>[3x]MNVASRVVVNADRVKGTINRNIYGHFSEHLGRCIYEGLWVGEDSPIPNTNGIRNDVLEALKQMKIPVLHWPGGCFADEYHWKDGVGPREKRKRMVNTHWGGVIEN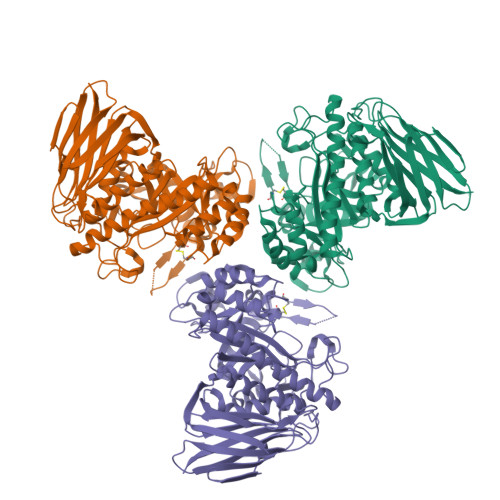NHFGTHEFMMLCELLGCEPYISGNVGSGTVQEMSEWVEYITFDGESPMANWRRENGREKPWRIKYWGVGNENWFCGGNMRAEYYADLYRQFQTYLRNYGDNKLHKIACGANTADYHWTEVLMKQAAPFMHGLSLHYYTVPGPWEKKGPATGFTTDEWWVTLKKALFMDRLVTKHSAIMDVYDPDKRIDLIVDEWGTWYDVEPGTNPGFLYQQNSIRDALVAGATLHIFHRHCDRVRMANIAQLVNVMQSVILTEGERMLLTPTYHVFNMFKVHQDAELLDTWESVERTGPEGELPKVSVSASRAADGKIHISLCNLDFETGASVDIELRGLNGGVSATGTTLTSGRIDGHNTFDEPERVKPAPFRDFKLEGGHLNASLPPMSVTVLELTAG> XTGMSGF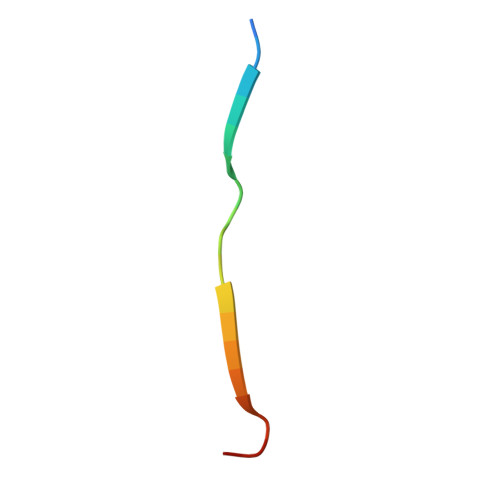SETVTIVEDTRPX>MKEVVIASAVRTAIGSYGKSLKDVPAVDLGATAIKEAVKKAGIKPEDVNEVILGNVLQAGLGQNPARQASFKAGLPVEIPAMTINKVCGSGLRTVSLAAQIIKAGDADVIIAGGMENMSRAPYLANNARWGYRMGNAKFVDEMITDGLWDAFNDYHMGITAENIAERWNISREEQDEFALASQKKAEEAIKSGQFKDEIVPVVIKGRKGETVVDTDEHPRFGSTIEGLAKLKPAFKKDGTVTAGNASGLNDCAAVLVIMSAEKAKELGVKPLAKIVSYGSAGVDPAIMGYGPFYATKAAIEKAGWTVDELDLIESNEAFAAQSLAVAKDLKFDMNKVNVNGGAIALGHPIGASGARILVTLVHAMQKRDAKKGLATLSIGGGQGTAILLEKCLEHHHHHH[2x]

Here, we present the crystal structure of C. acetobutylicum thiolase (CaTHL), a type II biosynthetic thiolase that catalyses the first step of n-butanol biosynthesis and condenses two acetyl-CoAs to acetoacetyl-CoA. We reveal that CaTHL, unlike other type II biosynthetic thiolases from aerobic bacteria, is regulated via modulation of a redox-switch, indicating that n-butanol production and the relevant metabolic fluxes in Clostridium are tightly regulated by thiolase. CaTHL consists of three domains: an N-terminal α/β domain (N-domain, residues 1–119 and 249–269), a loop domain (L-domain, residues 120–248), and a C-terminal α/β domain (C-domain, residues 270–392). The N- and C-domains form a typical five-layered fold (α–β–α–β–α) observed in other thiolase superfamily of proteins including peroxisomal degradative thiolase from Saccharomyces cerevisiae, β-ketoacyl synthase II from E. coli, and the biosynthetic thiolase from Zoogloea ramigera (ZrTHL)14151617181920.

Next, the crystal structure of the reduced form of CaTHL in complex with CoA was determined. The catalytic residues such as Cys88, Cys378 and His348 were observed to be located at the same positions as those of the corresponding residues of ZrTHL, indicating that the catalytic mechanism might be identical to that of ZrTHL. However, the CoA-binding mode of CaTHL was quite unique when compared with that of ZrTHL. In CaTHL, His218 residue, whose corresponding residue is Tyr218 in ZrTHL, is involved in the stabilization of pyrophosphate moiety of CoA, and Ser223 residue is located at the position of Ala223 in ZrTHL. Moreover, in CaTHL, Arg133 residue from the neighbouring polypeptide is involved in the stabilization of pyrophosphate moiety of CoA through hydrogen bond, whereas the corresponding Lys133 residue in ZrTHL has conformation distal from the bound CoA.>GPGWEKRTDPRGRFYYVDHNTRTTTWQRPTAEYVRNYEQWQSQRNQLQGAMQHFSQRFLYQSSSASQGSPGAYDRSFRWKYHQFRFLCHSNALPSHVKISVSRQTLFEDSFQQIMNMKPYDLRRRLYIIMRGEEGLDYGGIAREWFFLLSHEVLNPMYCLFEYAGKNNYCLQINPASSINPDHLTYFRFIGRFIAMALYHGKFIDTGFTLPFYKRMLNKRPTLKDLESIDPEFYNSIVWIKENNLEECGLELYFIQDMEILGKVTTHELKEGGESIRVTEENKEEYIMLLTDWRFTRGVEEQTKAFLDGFNEVAPLEWLRYFDEKELELMLCGMQEIDMSDWQKSTIYRHYTKNSKQIQWFWQVVKEMDNEKRIRLLQFVTGTCRL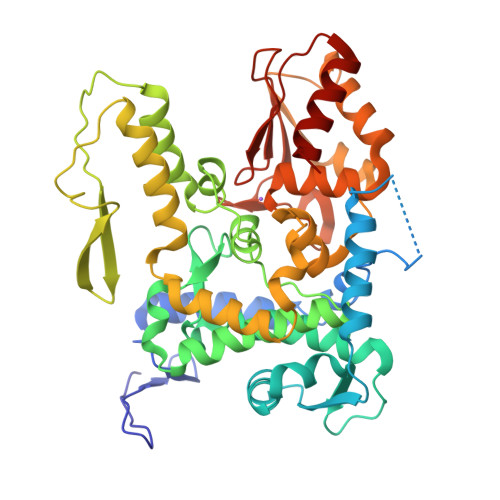PVGGFAELIGSNGPQKFCIDKVGKETWLPRSHTCFNRLDLPPYKSYEQLREKLLYAIEETE[4x]>[10x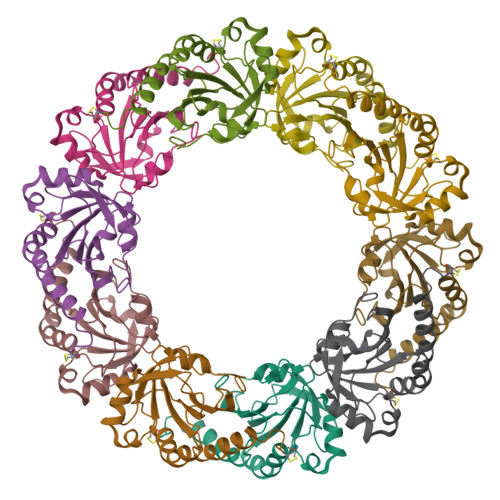]SLIGTEVQPFRAQAFQSGKDFFEVTEADLKGKWSIVVFYPADFSFVCPTELEDVQKEYAELKKLGVEVYSVSTDTHFVHKAWHENSPAVGSIEYIMIGDPSQTISRQFDVLNEETGLADRGTFIIDPDGVIQAIEINADGIGRDASTLINKVKAAQYVRENPGEVCPAKWEEGGETLKPSLDIVGKI>GSDKRGPQSAEPDPLERLEVKKVQQQHENEKDDSGRDTKSGGKVAKAMTKGDTIAGKLLTTPSRLFKLLIPLTTINRKDIEQIAILIHPQQPLSHLERLIQSEVPPIEDENGQKRPPFVSFIALQLEQDAIRPKRGMYEGTDAEIHRVEGGKDDATVAKRGEDFQEVDETFSYLRRPGPGQGDKEQRFIRWSQSTEIGDFIRDAARAKEFIVTIEGAPAGLEQIHVAVPSFDERTYFLRMRLRKISRRIQGLAEIKHECDALAHRGAQRVALGGFGILAFWWYIVYKLTFETDLGWDTMEPVTYLVSLSTLMGGYLWFLYHNREISYRSALDFTINARQKKLYQMKGIDLQV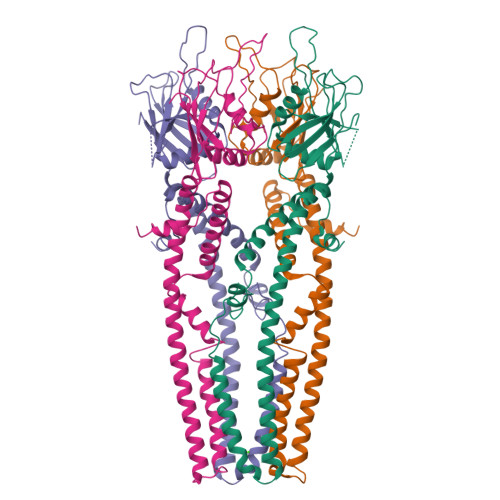WESLIDEANAIRREIKNIAAEYDVDWDERKDEQDDRVTEALKKERRLKNGSQKEERPKDDRDDD[4x]7-[(1S,5R)-1-amino-3-azabicyclo[3.1.0]hexan-3-yl]-4-(aminomethyl)-1-cyclopropyl-3,6-difluoro-8-methylquinolin-2(1H)-one 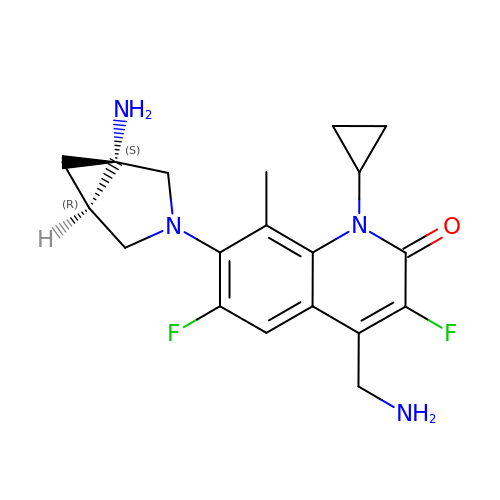| C19 H22 F2 N4 O | LZLLPIGCIXMSRM-GIGQVBGESA-N>[4x]AFLHVGKMGFVVTMLKLIQKKLLDKTCDQVMEFSWSALWNITDETPDNCEMFLNFNGMKLFLDCLKEFPEKQELHRNMLGLLGNVAEVKELRPQLMTSQFISVFSNLLESKADGIEVSYNACGVLSHIMFDGPEAWGVCEPQREEVEERMWAAIQSWDIN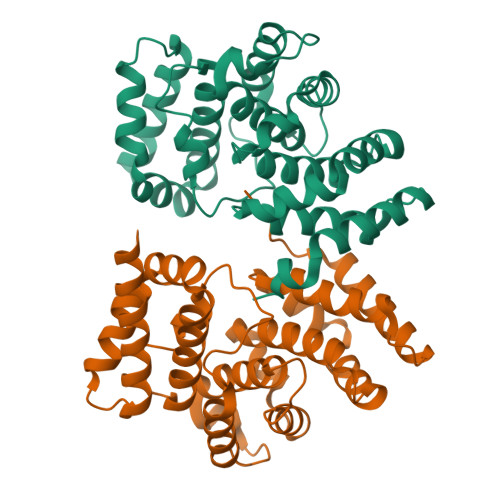SRRNINYRSFEPILRLLPQGISPVSQHWATWALYNLVSVYPDKYCPLLIKEGGMPLLRDIIKMATARQETKEMARKVIEHCSNFKEENMDTSR(2S)-(carbamoylamino)(hydroxy)ethanoic 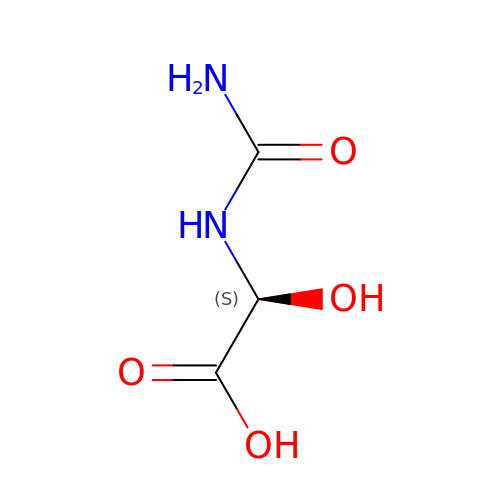acid | C3 H6 N2 O4 | NWZYYCVIOKVTII-SFOWXEAESA-N>GSGSG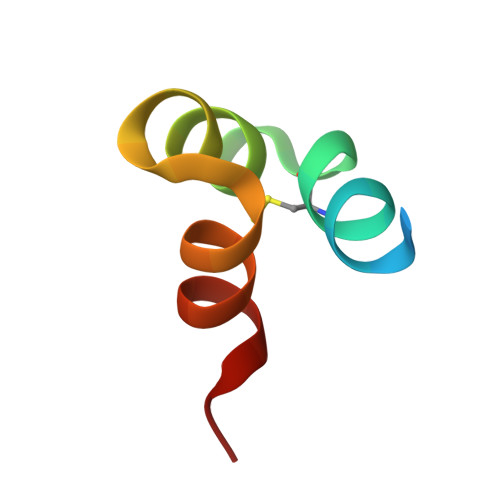EPKREVCELNPDCDELADHIGFQEAYRRFYGPV[2x]> MNKEEIILSAKNWMHSHFENETTGHDWSHIKRVWKLSKEIQSKEGGDLFTIELAALFHDYSDIKLTTDEQEATKTLINWMETKEIPSELIKKIIRIIQSVSFKKGKNTFKALTIEEKIVQDADRLDAIGAIGIARTF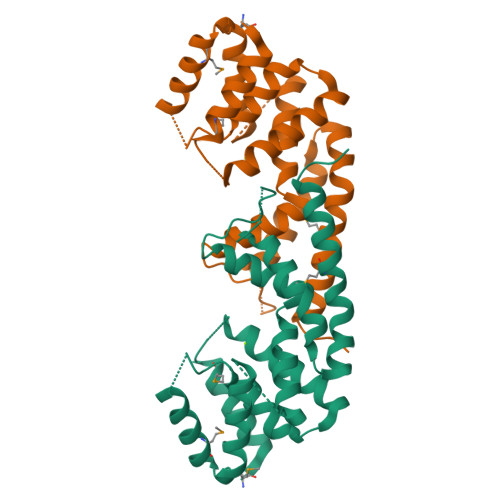TYGGAHNREIANQNNPKNTTLQHFYDKLLLIKDQLNTETAKTIAKEKQKIMQDFIQALEKELKVLEHHHHHH> MANEPQKSDDNGQAAEAVVTDDEIVLQDQQLKTIEDEQKSVPLVATLAPFSILCAEYDNETSAAFLSKATELSEVYGEIRYIRGDGNCFYRAILVGLIEIMLKDRARLEKFIASSRDWTRTLVELGFPDWTCTDFCDFFIEFLEKIHSGVHTEEAVYTILNDDGSANYILMFFRLITSAFLKQNSEEYAPFIDEGMTVAQYCEQEIEPMWKDADHLAINSLIKAAGTRVRIEYMDRTAAPNGGWHYDIPSDDQQIAPEITLLYRPGHYDVIYKKDSTEASEIEN;> MAGLPRRIIKETQRLLAEPVPGIKAEPDESNARYFHVVIAGPQDSPFEG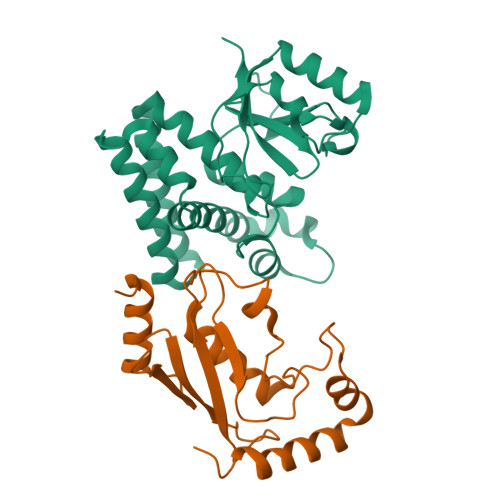GTFKLELFLPEEYPMAAPKVRFMTKIYHPNVDKLGRICLDILKDKWSPALQIRTVLLSIQALLSAPNPDDPLANDVAEQWKTNEAQAIETARAWTRLYAMNNI>GKLDATLRAIVHTAAELVDARYGALGVRGYD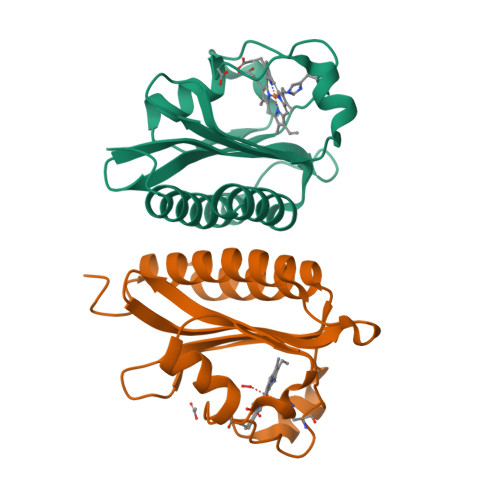HRLVEFVYEGIDEETRHLIGSLPEGRGVLGALIEEPKPIRLDDISRHPASVGFPLHHPPMRTFLGVPVRIRDEVFGNLYLTEKADGQPFSDDDEVLVQALAAAAGIAVDNARLFEESR[2x]Leukotriene A4 hydrolase (LTA4H) is an enzyme that classically functions as an epoxide hydrolase to generate leukotriene B4 (LTB4) from leukotriene A4 (LTA4)12. Recently, we identified a secondary anti-inflammatory activity for LTA4H whereby it functions as an aminopeptidases to degrade the tripeptide Pro-Gly-Pro (PGP). The enzyme itself is folded into 3 domains, which manifest as N-terminal, catalytic and C-terminal domains. The interface of these domains forms an L-shaped cavity where the active site of the enzyme is located.

We hypothesized that whilst conventional LTA4H inhibitors would occupy both sites it would be preferable to develop molecules to bind to one of the two overlapping binding sites (Site A) present in LTA4H, leaving Site B free to bind PGP. This should block detrimental hydrolase activity, whilst preserving beneficial peptidase function. The origins of the augmented capacity of compound 9 to inhibit LTA4H epoxide hydrolase activity were explored by modelling and X-ray crystallography. The X-ray structure of LTA4H shows high similarity to literature examples (RMSD between 606 atom pairs is 0.204 Å). Whilst 2H-resveratrol forms two interactions with Trp-311, one H-bond and one π-stack, these are absent in the compound 9 structure, where the 3-methoxy-5-phenol ring rotates to allow the phenol to H-bond to Asp-375. Importantly, previous site-directed mutational interrogation of the active site of the enzyme has identified Asp-375 to be the only residue uniquely and absolutely required for the enzyme’s epoxide hydrolase activity. This therefore likely underlies the far superior capacity of compound 9 versus 2H-resveratrol to inhibit that capacity of LTA4H to generate LTB4. Thus compound 9 represented a chemical series with clear and rational potential to selectively inhibit the epoxide hydrolase activity of LTA4H. Compound 9 exhibited sub-μM capacity to inhibit LTB4 generation in a cell based assay, whilst showing no inhibition of PGP degradation at 100 μM – thus exhibiting a superior selectivity to ARM1 in our hands. Whilst compound 9 exhibited a targeted potency and selectivity, preliminary studies suggest that it does not possess a suitable drug profile, being readily metabolized within microsomes.

> MPEIVDTCSLASPASVCRTKHLHLRCSVDFTRRTLTGTAALTVQSQEDNLRSLVLDTKDLTIEKVVINGQEVKYALGERQSYKGSPMEISLPIALSKNQEIVIEISFETSPKSSALQWLTPEQTSGKEHPYLFSQCQAIHCRAILPCQDTPSVKLTYTAEVSVPKELVALMSAIRDGETPDPEDPSRKIYKFIQKVPIPCYLIALVVGALESRQIGPRTLVWSEKEQVEKSAYEFSETESMLKIAEDLGGPYVWGQYDLLVLPPSFPYGGMENPCLTFVTPTLLAGDKSLSNVIAHEISHSWTGNLVTNKTWDHFWLNEGHTVYLERHICGRLFGEKFRHFNALGGWGELQNSVKTFGETHPFTKLVVDLTDIDPDVAYSSVPYEKGFALLFYLEQLLGGPEIFLGFLKAYVEKFSYKSITTDDWKDFLYSYFKDKVDVLNQVDWNAWLYSPGLPPIKPNYDMTLTNACIALSQRWITAKEDDLNSFNATDLKDLSSHQLNEFLAQTLQRAPLPLGHIKRMQEVYNFNAINNSEIRFRWLRLCIQSKWEDAIPLALKMATEQGRMKFTRPLFKDLAAFDKSHDQAVRTYQEHKASMHPVTAMLVGKDLKVDVDHHHHHH> MSQNQVPKWIQLNNEIMIQKDGKFQFDKDKEAVHSYFVDYINQNTVFFHNLKEKLDYLVENQYYEEEFLSLYSFEDIKEVFKTAYAKKFRFPSFMSAFKFYNDYALKTNDKKKILERYEDRISIVALFFANGDTEKAKEYVNLMINQEYQPSTPTFLNAGRKRRGELVSCFLLEVNDSLNDISRAIDISMQLSKLGGGVSLNLSKLRAKGEAIKDVENATKGVVGVMKLLDNAFRYADQMGQRQGSGAAYLNIFHRDINDFLDTKKISA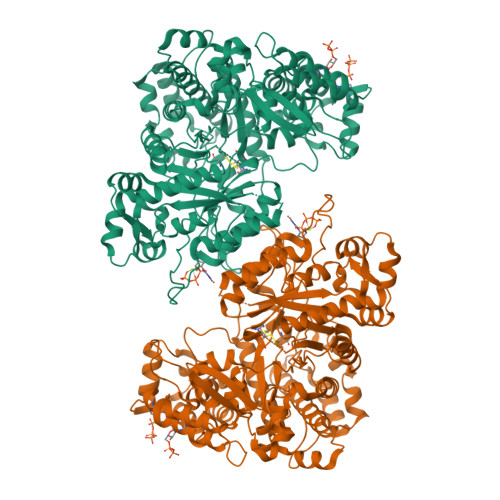DEDVRVKTLSIGVVIPDKFVELAREDKAAYVFYPHTIYKEYGQHMDEMDMNEMYDKFVDNPRVKKEKINPRKLLEKLAMLRSESGYPYIMFQDNVNKVHANNHISKVKFSNLCSEVLQASQVSSYTDYDEEDEIGLDISCNLGSLNILNVMEHKSIEKTVKLATDSLTHVSETTDIRNAPAVRRANKAMKSIGLGAMNLHGYLAQNGIAYESPEARDFANTFFMMVNFYSIQRSAEIAKEKGETFDQYEGSTYATGEYFDKYVSTDFSPKYEKIANLFEGMHIPTTEDWKKLKAFVAEHGMYHSYRLCIAPTGSISYVQSSTASVMPIMERIEERTYGNSKTYYPMPGLASNNWFFYKEAYDMDMFKVVDMIATIQQHIDQGISFTLFLKDTMTTRDLNRIDLYAHHRGIKTIYYARTKDTGQDSCLSCVV>MRGSHHHHHHGSLPVATMVSELIKENMPTKLYMEGTVNNHHFKCTSEGEGKPYEGTQTMRIKVVEGGPLPFAFDILATSFXSRTFIKHPPGIPDFFKQSFPEGFTWERVTTYEDGGVLTATQDTSLQDGCLIYNVKVRGVNFPSNGPVMQKKTLGWEASTETMYPADGGLEGRCDMALKLVGGGHLICNLKTTYRSKK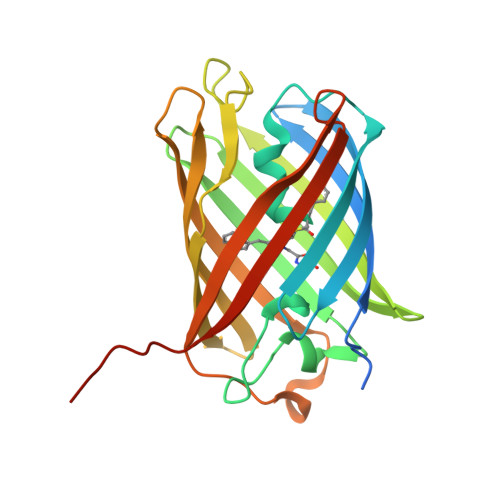PATKLKMPGVYYVDHRLERIKEADDETYVEQHEVAVARYCDLPSKLGHKLN[2x]>SQQLQKEEEARKVKSGIRQMRLFSQDECAKIEARIDEVVSRAEKGLYNEHTVDRAPLRNKYFFGEGYTYGAQLQKRGPGQERLYPPGDVDEIPEWVHQLVIQKLVEHRVIPEGFVNSAVINDYQPGGCIVSHVDPIHIFERPIVSVSFFSDSALCFGCKFQFKPIRVSEPVLSLPVRRGSVTVL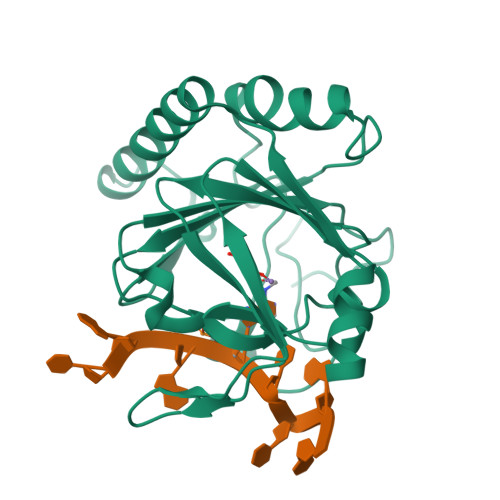SGYAADEITHCIRPQDIKERRAVIILRKTRLDAPRL[5x]> MSLHFLYYCSEPTLDVKIAFCQGFDKQVDVSYIAKHYNMSKSKVDNQFYSVEVGDSTFTVLKRYQNLKPIGSGAQGIVCAAYDAVLDRNVAIKKLSRPFQNQTHAKRAYRELVLMKCVNHKNIISLLNVFTPQKTLEEFQDVYLVMELMDANLCQVIQMELDHERMSYLLYQMLCGIKHLHSAGIIHRDLKPSNIVVKSDCTLKILDFGLARTAGTSFMMTPYVVTRYYRAPEVILGMGYKENVDIWSVGCIMGEMVRHKILFPGRDYIDQWNKVIEQLGTPCPEFMKKLQPTVRNYVENRPKYAGLTFPKLFPDSLFPADSE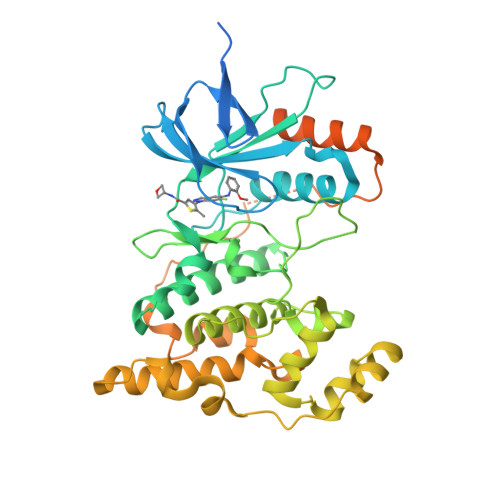HNKLKASQARDLLSKMLVIDPAKRISVDDALQHPYINVWYDPAEVEAPPPQIYDKQLDEREHTIEEWKELIYKEVMNSEEKTKNGVVKGQPSPSGAAVNSSESLPPSSSVNDISSMSTDQTLASDTDSSLEASAGPLGCCR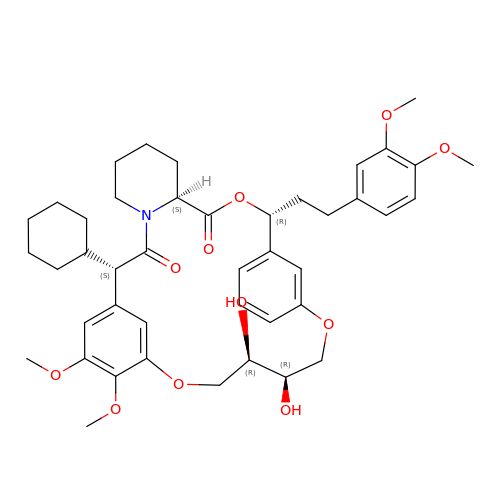2-cyclohexyl-12-[2-(3,4-dimethoxyphenyl)ethyl]-20,21-dihydroxy-25,26-dimethoxy-11,18,23-trioxa-4-azatetracyclo[22.3.1.113,17.04,9]nonacosa-1(27),13(29),14,16,24(28),25-hexaene-3,10-dione | C43 H55 N O11 | KMMZNLFAOHLXKG-NXKLTUDVSA-N>MGAFAPHFGSPFVRTSDYGKRPGLYGDFHTGIDYAAPTGTPIPAQYPGLVDWVQSSSIGLGEHVGIKVADNLWAMYGHMSRIRAKMGDKVKAGQIVGDVGSSGWSTGPAVHYELRKGGPNGQHVNPDTYGGAAGGSHHHHHH[5x]

EnpA is a prophage encoded 1721 residues protein composed of three domains; the N-terminal domain (1350 amino acids) shares homology with phage tail tape measure proteins. The two domains located towards the C-terminus of EnpA are homologous to domains belonging to PG hydrolases with lytic transglycosylase activity (cleaving glycan chains) and M23 peptidase activity (cleaving PG peptides). The functional analysis of the EnpA catalytic domain (EnpACD) revealed its hydrolytic activity on the D-Ala–L-Ala bond, which is characteristic for E. faecalis peptidoglycan, and proposed the minimum substrate of EnpCD to consist of three residues of the donor stem and the amino acids of the cross-bridge. Members of the M23 family are metallopeptidases containing a zinc ion in their active site, coordinated by two histidine and one aspartic acid residues in the conserved motifs: HXXXD and HXH.

Despite multiple attempts to crystallize and solve the EnpACD structure, we were unable to obtain crystals of the wild-type protein diffracting below 4 Å; therefore, we generated an inactive variant of EnpACD H109A. The crystals of this variant gave better diffraction data that were then used to solve the structure of EnpACD at a resolution of 3 Å. The crystal structure revealed five protein molecules in the asymmetric unit (ASU). All EnpACD molecules in the ASU are similar with root-mean-square deviation (RMSD) values of 0.35 Å–0.65 Å and β-factors for chains A–E ranging from 87 to 108 Å2. EnpACD is a globular all β-structure molecule that could be divided into two β-sheets. A central β-sheet creates the bottom of the active site groove while its walls are restricted by three out of four protruding loops, as loop 4 rather sticks to the protein core. The organization of the active site is conserved among the members of the enzymatically active peptidoglycan hydrolases from the M23 family, and a strong electron density corresponding to a metal ion was observed in the close vicinity of His29, Asp33 and His111, residues coordinating Zn2+. EnpACD substrate pocket is placed on the plane of the central β-sheet, and its walls are defined by loops that build a deep (10–20 Å) and very narrow (4–5 Å) groove. In the EnpACD structure, the Arg21 side chain is in close contact with Ser16 and Asp27, suggesting the formation of the hydrogen bond and a salt bridge. The EnpA broader specificity is achieved by opening the binding groove at the prime site making it more accessible for a wider range of substrates.> MNFNVSLMEKLKWKIKCIENKFLNYRLTTNETVVAETEYGKVKGVKRLTVYDDSYYSFEGIPYAQPPVGELRFKAPQRPTPWDGVRDCCNHKDKSVQVDFITGKVCGSEDCLYLSVYTNNLNPETKRPVLVYIHGGDFIIGENHRDMYGPDYFIKKDVVLINIQYRLGALGFLSLNSEDLNVPGNAGLKDQVMALRWIKNNCANFGGNPDNITVFGESAGAASTHYMMLTEQTRGLFHRGILMSGNAICPWANTQCQHRAFTLAKLAGYKGEDNDKDVLEFLMKAKPQDLIKLEEKVLTLEERTNKVVFPFGPTVEPYQTADCVLPKHPREMVKTAWGNSIPTMMGNTSYEGLFFTSILKQMPMLVKELETCVNFVPSELADVERTAPETLEMGAKIKKAHVTGETPTADNFMDLCSHIYFWFPMHRLLQLRFNHTSGTPVYLYRFDFDSEDLINPYRIMRSGRGVKGVS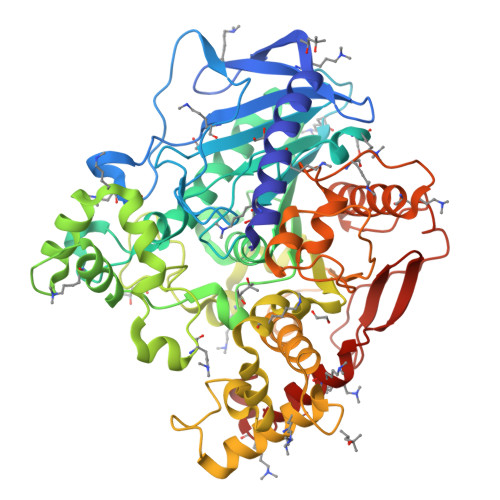HADELTYFFWNQLAKRMPKESREYKTIERMTGIWIQFATTGNPYSNEIEGMENVSWDPIKKSDEVYKCLNISDELKMIDVPEMDKIKQWESMFEKHRDLF> MGSSHHHHHHLEVLFQGPAGSMATERDQEIIDFIDQGNYTYAQSLITKKLAKSPQKLFYHVLQNEIHLKSGQRELAIKKNLELLNRYPNDPLTIEKLSDFFSKMEMEKESSLVYENAIKKYPVSTETLCLSWFDNSIEKYDFKVFNRIFMYLNKNGKSRLHTLWYAFSFHLLLQEGETDKASLYNSLGKKLMEGLQPFENTQEIYVYTLFLSSKEIEQVLSGVTLPLDLELKLLYMKAMKENASFEALHAYTEKLLFKEKFDDFDTWKLWILSGKEIGKSFEELDQKLTLPTRNISLLKIELDILYSRNIETSVENYYQKFNTKLCCYADLSQYELPTSFIGSLKNSTSEENLITVVNNRKFVNQTDNWDVYERFSTKEGAEYDSNPVNELTLRTIVSDLDSSPQNTIKNIVLLKHLLEQDKYNYKLKLWLMKLYSQLNTNDLIFPIYNGLKIRMTQH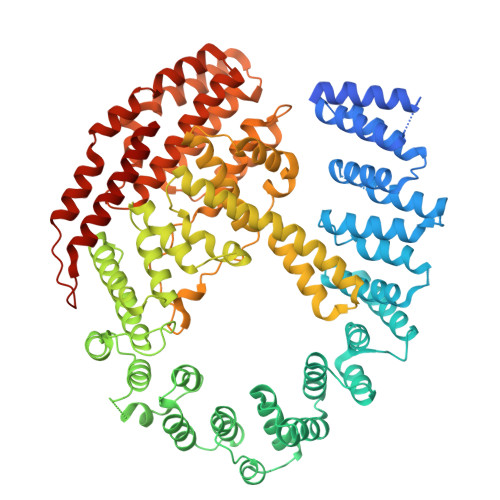ETLNYYLTTTNPSKINLDAWVDIYRFYLTSKQEIKESIIQGFDNGVFNKLEGFINFSKRMQNSISLNFTVAKILQISTILGTDGYLNYFIHYLKTNEALIVSDYTDNRDFKSEWNGLEKIDCIDVPVNDVATKLKLLVYSIVFEDQDASRLLKVFNKITSNAKFSVFDNLLYKLYFNLLKITKTKLNPQETQSLYNYLQKNLKTDKLKILIPENLLSGELTQNLTNLVEFIKIVKLLAKRHPSSYMNQLVNLVKPFGKEFKNLKLVQRQHEIIDSMDFEPPISVDISQTKLEIKSSIEDCVVALLNSL2-(4-fluorophenyl)-~{N}-[(4-phenoxyphenyl)methyl]ethanamine | C21 H20 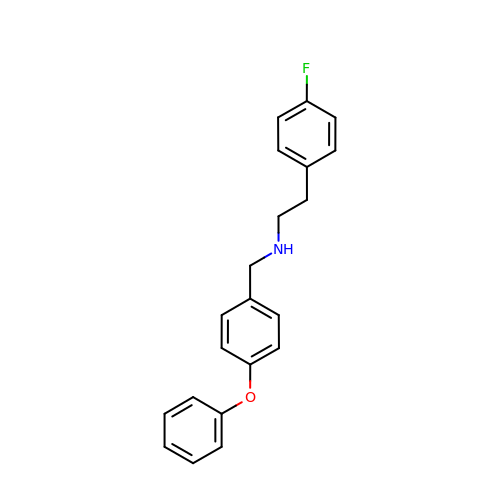F N O | BPPBYUPUAFZCNN-UHFFFAOYSA-N>[6x]MNAQAEEFKKYLETNGIKPKQFHKKELIFNQWDPQEYCIFLYDGITKLTSISENGTIMNLQYYKGAFVIMSGFIDTETSVGYYNLEVISEQATAYVIKINELKELLSKNLTHFFYVFQTLQKQVSYSLAKFNDFSINGKLGSICGQLLILTYVYGKETPDGIKITLDNLTMQELGYSSGIAHSSAVSRIISKLKQEKVIVYKNSCFYVQNLDYLKRYAPKLDEWFYLACPATWGKLN

In relation to pathogenesis, the expression of most virulence genes in L. monocytogenes is regulated by the master regulator PrfA, which is a member of the Crp/Fnr family of site-specific DNA-binding transcription regulators. PrfA activates transcription by binding to a palindromic promoter element termed the PrfA box (tTAACanntGTtAa). Very recently, glutathione (GSH), either generated by bacteria or derived from host cells, was found to be the essential small molecule cofactor of PrfA through allosteric binding to the protein. In this study, we determined the crystal structures of PrfA-DNA binary and PrfA-DNA-GSH ternary complexes, thereby providing new insights into the mechanism of PrfA-mediated gene regulation.

The complex contains one PrfA dimer bound to one dsDNA molecule and exhibits an intramolecular 2-fold pseudosymmetry. Each PrfA monomer consists of an N-terminal domain (aa 1–108), a long α-helical linker (aa 109–1137), and a helix-loop-helix-containing C-terminal domain (aa 138–1237). The overall DNA bend is ~45° in the PrfA-DNA complex, which is significantly different from the previously reported bend values of approx. 80° to 90° for Crp-DNA and CprK-DNA complexes. The intermolecular contacts between PrfA dimer and DNA contain both specific interactions with bases and nonspecific interactions with sugar-phosphate backbone. The second helix of the helix-loop-helix motif penetrates into the major groove of the DNA, with S184 and R188 forming direct hydrogen bonds with the bases of T20 and G18, respectively. The majority of the intermolecular contacts are between PrfA and the sugar-phosphate backbone of the DNA. We observed a DNA-induced conformational change of PrfA by comparing the structures of PrfA in free and DNA bound states. The conformation of PrfA in the PrfA-DNA and PrfA-DNA-GSH complexes is similar to the constitutively active mutant PrfAG145S in free state, consistent with the previous prediction that PrfAG145S mutant adopts an induced conformation. However, we did not observe conformational differences between the PrfA-DNA binary complex and the PrfA-DNA-GSH ternary complex, which is consistent with the previous understanding that PrfA could interact with DNA in vitro even in the absence of an activator.>[14x]XGELAQSIKELAKSIKEEAWSIKELAQSIKGX

CCs are quaternary structures comprising two or more α-helices supercoiled around each other with cyclic (Cn) or dihedral (Dn) symmetry. Here, we describe variants with all combinations of the aliphatic residues, Ile, Leu and Val, at a and d to give four classes of peptide: the ββ class, with a and d = Ile or Val; Lβ, a = Leu and d = Ile or Val; βL, a = Ile or Val and d = Leu; and LL, a = d = Leu. Peptides are named systematically appending the one-letter code for the amino acids at the a and d sites to “CC-Type2-“; e.g., CC-Hept becomes CC-Type2-LI. In summary, solution-phase data and X-ray crystal structures demonstrate conclusively that different classes of Type-2 coiled-coil (CC) peptides—i.e., based on abcdefg repeats with predominantly hydrophobic residues at a, d, e and g—adopt a range of distinct states.

To explore this switch between assembling open α-helical barrels and collapsed CCs, we tested if examples of some of the latter could be opened by introducing polar residues into the hydrophobic repeats of βL and LL sequences. Specifically, we mutated the centremost Leu at d (position 17) to Glu to give CC-Type2-IL-Sg-L17E and CC-Type2-LL-L17E. However, unlike the parents, they had accessible thermal unfolding transitions. Both transitions were pH dependent with stabilities increasing sharply below pH 6–7. Neither of the L17E peptides bound DPH, but both sequestered its cationic derivative trimethyl-ammonium DPH (TMA-DPH) with μM affinities suggesting that the barrel states are accessible. Thus, L17E expands the collapsed hexamer of CC-Type2-IL to include a seventh helix and to reveal an accessible central channel. The experiments and calculations for CC-Type2-IL-Sg-L17E were similar; although, as expected for an open barrel, for a given charge state the macroscopic pKa values were lower than for the collapsed structure of CC-Type2-LL-L17E. For CC-Type2-IL-Sg-L17E, the central cavity was hydrated throughout the simulation. Thus, both the IL and LL backgrounds can switch and open to access barrel states. Moreover, this state appears to be more accessible to IL, fitting our contention that β-branched residues at a and d promote the α-helical-barrel state.METHYL (2S)-[1-((N-(NAPHTHALENEACETYL))-L-VALYL)AMINOMETHYL)HYDROXYPHOSPHINYLOXY]-3-PHENYL 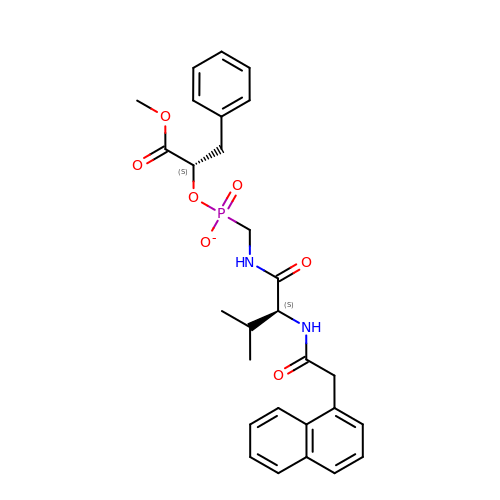PROPANOATE | C28 H32 N2 O7 P | AYDPZCGMCQBSDG-AHWVRZQESA-M> REEYD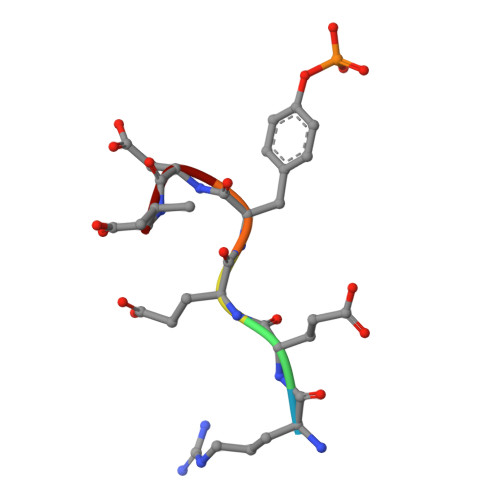V>GSAAPESLSPGATAEEAPEEDEDDAEAEDPERG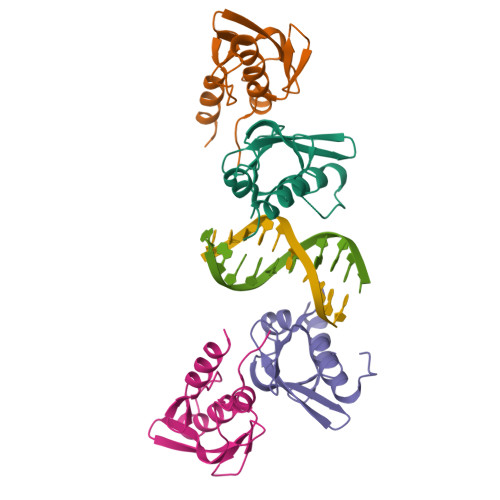TGSGGRSGSLGGSGGGTAGPGMALGGALTRRAVTLRVLLKDELLEPGEGVLSIYYLGRKFTGDLQLDGRIVWQETGQVFNSPSAWATHCKKLVNPAKKSGCGWASVKYKGQKLDKYKAAWLRRHQLHM[4x]> GPGSSLSRFRGCLAGALLGDCVGSFYEAHDTVDLTSVLRHVQSLEPDPGTPGSERTEALYYTDDTAMARALVQSLLAKEAFDEVDMAHRFAQEYKKDPDRGYGAGVVTVFKKLLNPKCRDVFEPARAQFNGKGSYGNGGAMRVAGISLAYSSVQDVQKFARLSAQLTHASSLGYNGAILQALAVHLALQGESSSEHFLKQLLGHMEDLEGDAQSVLDARELGMEERPYSSRLKKIGELLDQASVTREEVVSELGNGIAAFESVPTAIYCFLRCMEPDPEIPSAFNSLQRTLIYSISLGG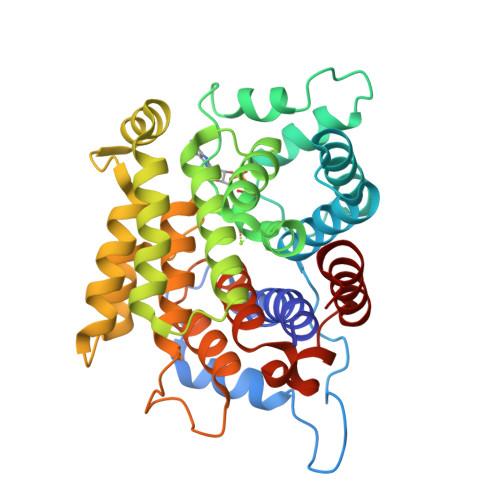DTDTIATMAGAIAGAYYGMDQVPESWQQSCEGYEETDILAQSLHRVFQKS> ATIEVRNNCPYTVWAASTPIGGGRRLNRGQTWVINAPRGTKMARIWGRTGCNFNAAGRGTCQTGDCGGV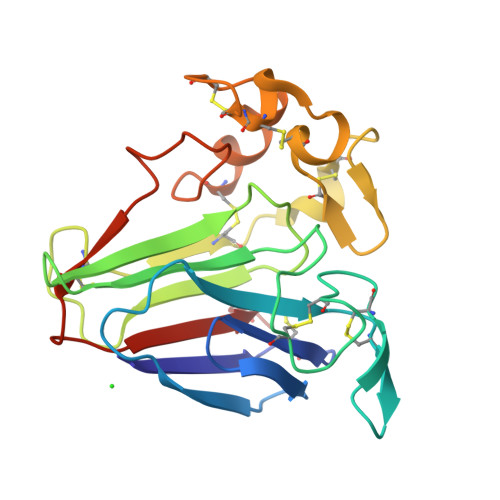LQCTGWGKPPNTLAEYALDQFSNLDFWDISLVDGFNIPMTFAPTKPSGGKCHAIHCTANINGECPRALKVPGGCNNPCTTFGGQQYCCTQGPCGPTELSKFFKKRCPDAYSYPQDDPTSTFTCPGGSTNYRVVFCPNG5-{2-[1-(5-HYDROXY-1,5-DIMETHYL-HEXYL)-7A-METHYL-OCTAHYDRO-INDEN-4-YLIDENE]-ETHYLIDENE}-2-METHYLENE-CYCLOHEXANE-1,3-DIOL 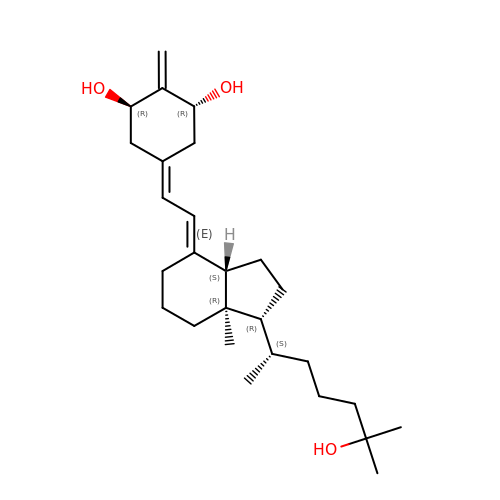| C27 H44 O3 | UHMPCVGLSKFXHR-NAQZCRMNSA-N~{N}-(3-azanyl-4-chloranyl-phenyl)-2-methoxy-ethanamide | C9 H11 Cl N2 O2 | 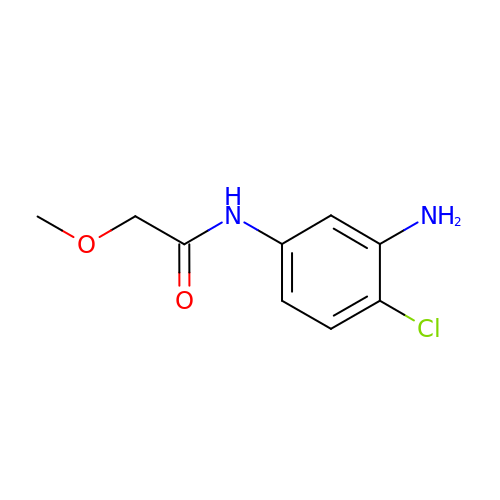NBKYWFKVWBQTFN-UHFFFAOYSA-N> GGACGATC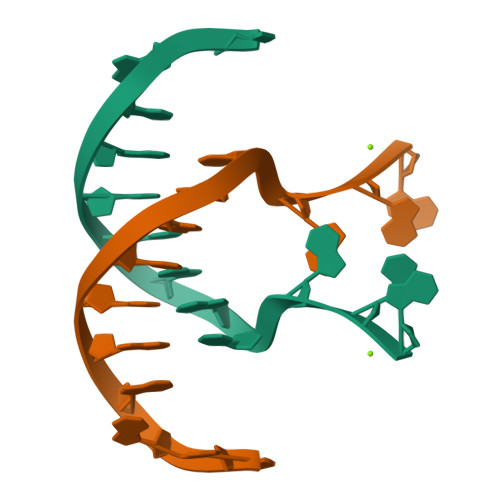GGGAG> TQFAFVFPG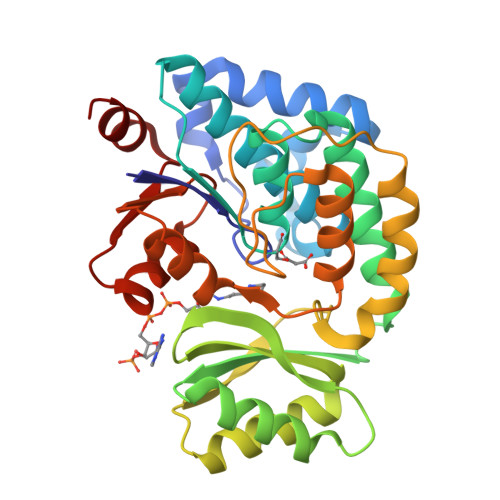QGSQTVGMLADMAASYPIVEETFAEASAALGYDLWALTQQGPAEELNKTWQTQPALLTASVALYRVWQQQGGKAPAMMAGHSLGEYSALVCAGVIDFADAVRLVEMRGKFMQEAVPEGTGAMAAIIGLDDASIAKACEEAAEGQVVSPVNFNSPGQVVIAGHKEAVERAGAACKAAGAKRALPLPVSVPSHCALMKPAADKLAVELAKITFNAPTVPVVNNVDVKCETNGDAIRDALVRQLYNPVQWTKSVEYMAAQGVEHLYEVGPGKVLTGLTKRIVDTLTASALNEPSAMAAALEL>[2x]MGSSHHHHHHSSGLMITPIISSNLGLKHRVTLRKATLASLMQSLSGESSNRVMWNDRYDTLLIARDPREIKNAIEKSVTDFGGLENYKELTGGADPFALMTPVCGLSANNIFKLMTEKDVPIDPTSIEYLENTSFAEHVNTLDSHKNYVVIVNDGRLGHKFLIDLPALTQGPRTAYIIQSDLGGGALPAVRVEDWISRRGSDPVSLD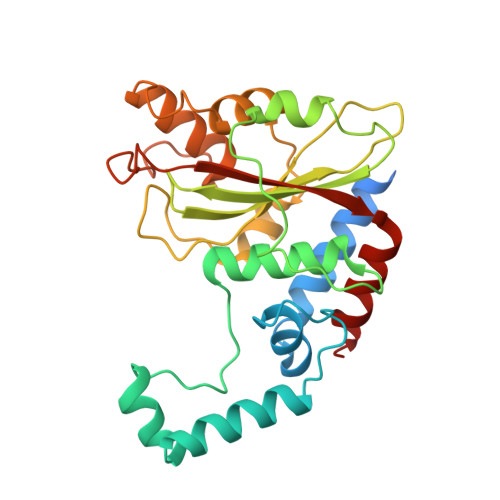ELNQLLSKDFSKMPDDVQTRLLASILQIDKDPHKVDIKKLHLDGKLRFASHEYDFRQFQRNAQYVAGLG> MSNFAIILAAGKGTRMKSDLPKVLHKVAGISMLEHVFRSVGAIQPEKTVTVVGHKAELVEEVLAEQTEFVTQSEQLGTG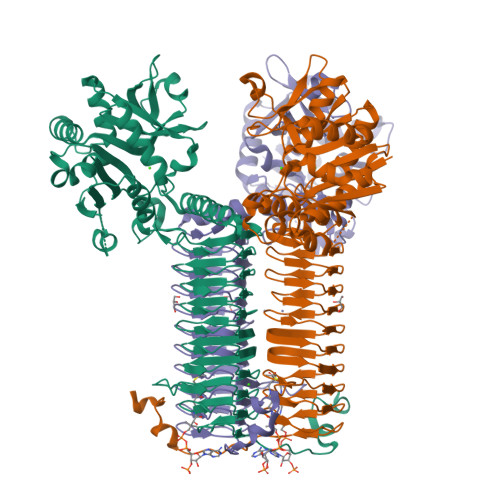HAVMMTEPILEGLSGHTLVIAGDTPLITGESLKNLIDFHINHKNVATILTAETDNPFGYGRIVRNDNAEVLRIVEQKDATDFEKQIKEINTGTYVFDNERLFEALKNINTNNAQGEYYITDVIGIFRETGEKVGAYTLKDFDESLGVNDRVALATAESVMRRRINHKHMVNGVSFVNPEATYIDIDVEIAPEVQIEANVILKGQTKIGAETVLTNGTYVVDSTIGAGAVITNSMIEESSVADGVTVGPYAHIRPNSSLGAQVHIGNFVEVKGSSIGENTKAGHLTYIGNCEVGSNVNFGAGTITVNYDGKNKYKTVIGDNVFVGSNSTIIAPVELGDNSLVGAGSTITKDVPADAIAIGRGRQINKDEYATRLPHHPKNQ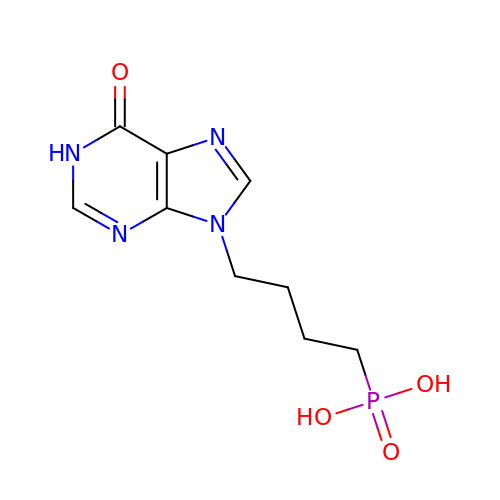4-(6-oxidanylidene-1~{H}-purin-9-yl)butylphosphonic acid | C9 H13 N4 O4 P | SXKIHSHTTWSCGF-UHFFFAOYSA-N> ESSVTLFGIVDTNVAYVNKDAAGDSRYGLGTSGASTSRLGLRGTEDLGGGLKAGFWLEGEIFGDDGNASGFNFKRRSTVSLSGNFGEVRLGRDLVPTSQKLTSYDLFSATGIGPFMGFRNWAAGQGADDNGIRANNLISYYTPNFGGFNAGFGYAFDEKQTIGTADSVGRYIGGYVAYDNGPLSASLGLAQQKTAVGGLATDRDEITLGASYNFGVAKLSGLLQQTKFKRDIGGDIKTNSYMLGASAPVGGVGEVKLQYALYDQKAIDSKAHQITLGYVHNLSKRTALYGNLAFLKNKDASTLGLQAKGVYAGGVQAGESQTGVQVGI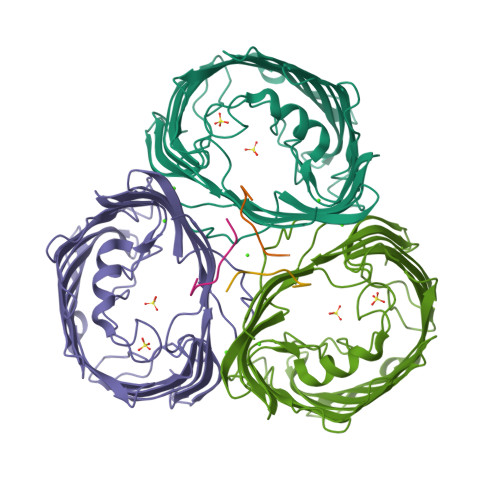RHAF;> DNWQNGTS>MKIAVIGQSLFGQEVYCQLRKEGHEVVGVFTIPDKDGKADPLGLEAEKDGVPVFKFPRWRARGQALPEVVAKYQALGAELNVLPFCSQFIPMEVINAPRHGSIIYHPSLLPRHRGASAINWTLIHGDKKGGFTIFWADDGLDTGDLLLQKECEVLPDDTVSTLYNRFLFPEGIKGMVQAVRLIAEGTAPRCPQSEEGATYEGIQKKETAKINWDQPAEAIHNWIRGNDKVPGAWTEACGQKLTFFNSTLNTSGLSTQGEALPIPGAHRPGVVTKAGLILFGNDDRMLLVKNIQLEDGKMMPASQFFKGSASSSLELTEAELATAEAVRSSWMRILPNVPEVEDSTDFFKSGAASVDVVRLVEEVKELCDGLELENEDVYMATTFRGFIQLLVRKLRGEDDESECVINYVEKAVNKLTLQMPYQLFIGGEFVDAEGSKTYNTINPTDGSVICQVSLAQVSDVDKAVAAAKEAFENGLWGKINARDRGRLLYRLADVMEQHQEELATIEALDAGAVYTLALKTHVGMSIQTFRYFAGWCDKIQGATIPINQARPNRNLTLTKKEPVGVCGIVIPWNYPLMMLSWKTAACLAAGNTVVIKPAQVTPLTALKFAELTLKAGIPKGVVNILPGSGSLVGQRLSDHPDVRKIGFTGSTEVGKHIMKSCALSNVKKVSLELGGKSPLIIFADCDLNKAVQMGMSSVFFNKGENCIAAGRLFVEESIHNQFVQKVVEEVEKMKIGNPLERDTNHGPQNHEAHLRKLVEYCQRGVKEGATLVCGGNQVPRPGFFFQPTVFTDVEDHMYIAKEESFGPIMIISRFADGDVDAVLSRANATEFGLASGVF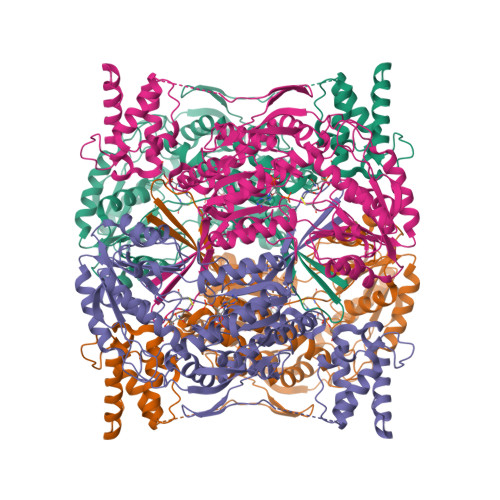TRDINKALYVSDKLQAGTVFINTYNKTDVAAPFGGFKQSGFGKDLGEAALNEYLRIKTVTFEY[4x]> MNGIHDVGGMDGFGKIM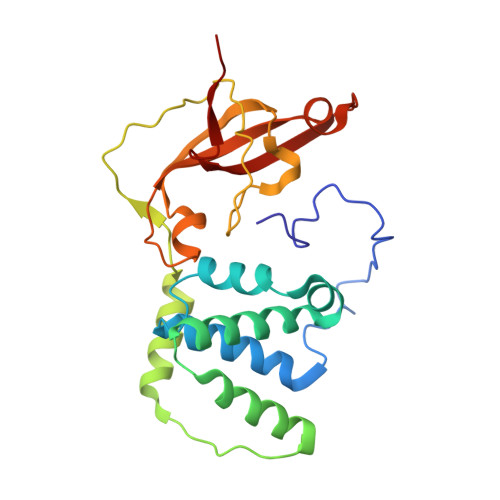YVKEEEDTYFKHDWERLTFGLVAGCMAQGLGMKAFDEFRIGIEKMRPVDYLTSSYYGHWIATVAYNLLETGVLDEKELEDRTQAFMEKPDTKIQRWENPKLVKVVEKALLEGLSPVREVSSFPRFEVGERIKTRNIHPTGHTRFPRYVRDKYGVIEEVYGAHVFPDDAAHRKGENPQYLYRVRFDAEELWGVKQNDSVYIDLWEGYLEPVSH Homologous recombination appears to be essential in the repair of double-stranded DNA breaks and the restarting of stalled replication forks. These proteins facilitate a pivotal DNA strand-exchange process between a single-stranded DNA (ssDNA) and a homologous double-stranded DNA (dsDNA) in homologous recombination. Here, we report the first crystal structure of hexameric RadA from Methanococcus voltae devoid of its first 60 amino-acid residues (Δ60MvRadA). The Δ60MvRadA protein is composed solely of the conserved ATPase domain found in RecA orthologues.

Similar to the previously studied Δ62MvRadA, Δ60MvRadA is active in hydrolyzing ATP in the presence of poly(dT)36 but inactive in promoting DNA strand exchange (data not shown). The ATP-binding P-­loop (residues Gly105–Thr112) was ordered with two putative nitrate ions, consistent with the requirement for a high concentration of sodium nitrate in the crystallization solution. The peptide chain was largely ordered except for residues 261–268 in the DNA-interacting L2 region (residues Asn256–Arg285). The central channel is lined by L1 regions (residues Arg218–Arg230) and has a diameter of 10 Å. Each L1 region has three conserved arginine residues (Arg218, Arg224 and Arg230 in MvRadA) in RadA/Rad51/DMC1 proteins. As a result, the central channels of such assemblies are highly positively charged. The conformation of each RadA monomer in the hexameric form clearly resembles the ATPase-active form. A short helix (residues Gly275–Ala282) was observed in the L2 region which corresponds to helix G in EcRecA. The conformational similarity of Δ60MvRadA and the ATPase-active form of MvRadA in the helix G region suggests that this short helix is inherently stable. Unlike the structures of filamentous MvRadA, the hexameric Δ60MvRadA structure revealed a different conformation of Arg74 which is no longer capable of retaining the salt bridge to Glu96.

>[6x]GSHMDLGFKSGIDLLKQRSTVWKLSTSSSELDSVLGGGLESQSVTEFAGVFGSGKTQIMHQSCVNLQNPEFLFYDEEAVSKGEVAQPKAVYIDTEGTFRPERIMQMAEHAGIDGQTVLDNTFVARAYNSDMQMLFAEKIEDLIQEGNNIKLVVIDSLTSTFRNEYTGRGKLAERQQKLGRHMATLNKLADLFNCVVLVTNQVSAKPDAFFGMAEQAIGGHIVGHAATFRFFVRKGKGDKRVAKLYDSPHLPDAEAIFRITEKGIQD> MKDLSEAQVER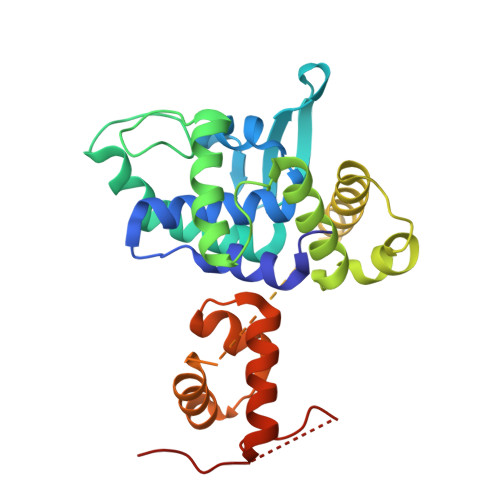LLQAPLIDQPLELRDKAMLEVLYATGLRVSELVGLTMSDISLRQGVVRVIGKGNKERLVPLGEEAVYWLETYLEHGRPWLLNGVSIDVLFPSQRAQQMTRQTFWHRIKHYAVLAGIDSEKLSPHVLRHAFATHLLNHGADLRVVQMLLGHSDLSTTQIYTHVATERLRQLHQQHHPRAGGGSEGGGSEGGSGSRTGAEELDPLFDQAVQFVTEKRKASISGVQRQFRIGYNRAARIIEQMEAQGIVSEQGHNGNREVLAPPPFD>[2x]PGCNKTNDHFTMQPGVNFYTVPNLGPSSSSADECYTNPSFSIGSSIYMFSQEIRKTDCTTGEILSIQIVLGRIVDKGQQ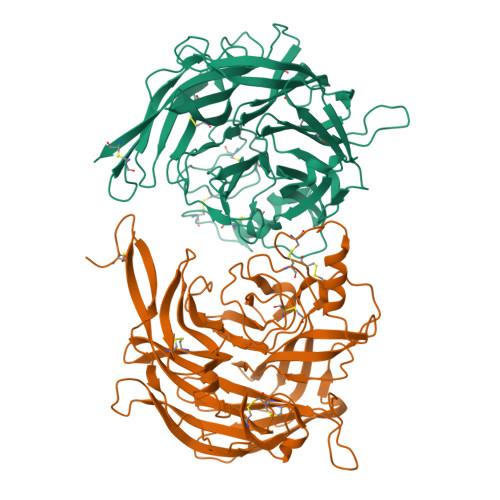GPQASPLLVWSVPNPKIINSCAVAAGDETGWVLCSVTLTAASGEPIPHMFDGFWLYKFEPDTEVVAYRITGFAYLLDKVYDSVFIGKGGGIQRGNDLYFQMFGLSRNRQSIKALCEHGSCLGTGGGGYQVLCDRAVMSFGSEESLISNAYLKVNDVASGKPTIISQTFPPSDSYKGSNGRIYTIGERYGIYLAPSSWNRYLRFGLTPDISVRSTTWLKEKDPIMKVLTTCTNTDKDMCPEICNTRGYQDIFPLSEDSSFYTYIGITPSNEGTKSFVAVKDDAGHVASITILPNYYSITSATISCFMYKEEIWCIAVTEGRKQKENPQRIYAHSYRVQKMCFHHHH> T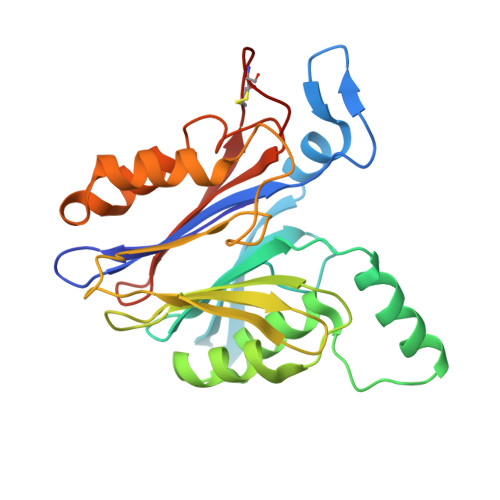ICTSIVAEDKKGHLIHGRNMDFGVFLGWNINNDTWVITEQLKPLTVNLDFQRNNKTVFKASSFAGYVGMLTGFKPGLFSLTLNERFSINGGYLGILEWILGKKDAMWIGFLTRTVLENSTSYEEAKNLLTKTKILAPAYFILGGNQSGEGCVITRDRKESLDVYELDAKQGRWYVVQTNYDRWKHPFFLDDRRTPAKMCLNRTSQENISFETMYDVLSTKPVLNKLTVYTTLIDVTKGQFETYLRDCPDPCIGW> GHMSQPLNVAVVGATGSVGEALVGLLDERDFPLHRLHLLASAESAGQRMGFAESSLRVGDVDSFDFSSVGLAFFAAAAEVSRAHAERARAAGCSVIDLSGALEPSVAPPVMVSVNAERLASQAAPFLLSSPCAVAAELCEVLAPLLATLDCRQLNLTACLSVSSLGREGVKELARQTAELLNARPLEPRLFDRQIAFNLLAQVGAVDAEGHSAIERRIFAEVQALLGERIGPLNVTCIQAPVFFGDSLSVTLQCAEPVDLAAVTRVLDATKGIEWVGEGDYPTVVGDAL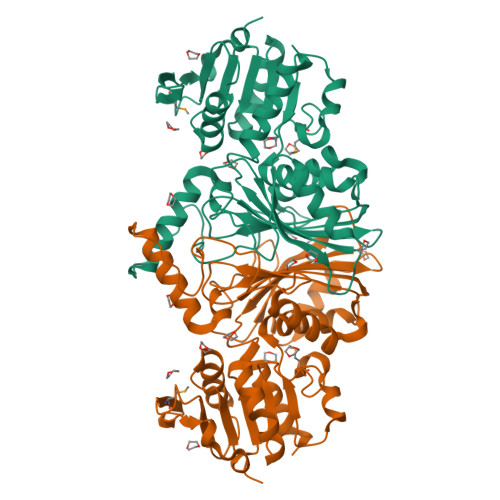GQDETYVGRVRAGQADPCQVNLWIVSDNVRKGAALNAVLLGELLIKHYLGS N-{[3-(4-amino-2-methylquinazolin-7-yl)phenyl]sulfonyl}-L-threoninamide | C19 H21 N5 O4 S | 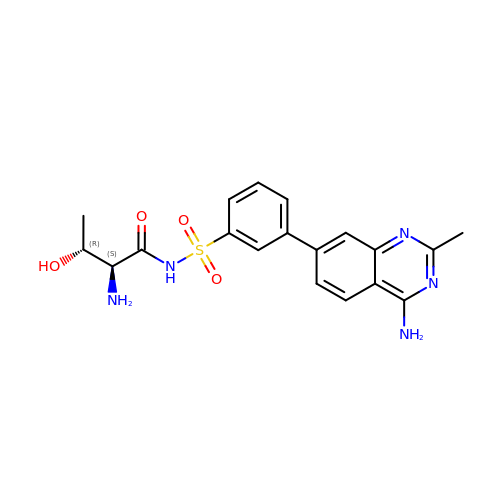CTJLRNBGVURJQO-QGHHPUGFSA-N>[3x]GDIIWDQLIVKR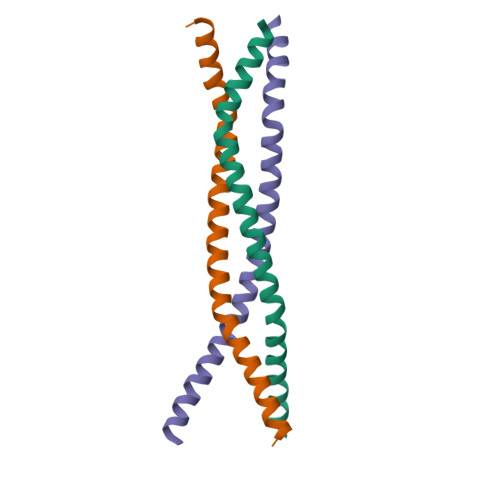TLADLLIPINRQISDIQSTLSEVTTRVHEIERQLHEITPVLKMGRTLEAISKGMSEMLAK> MAPKAKIVLVGSGMIGGVMATLIVQKNLGDVVLFDIVKNMPHGKALDTSHTNVMAYSNCKVSGSNTYDDLAGADVVIVTAGFTKAPGKSDKEANRDDLLPLNNKIMIEIGGHIKKNCPNAFIIVVTNPVDVMVQLLHQHSGVPKNKIIGLGGVLDTSRLKYYISQKLNVCPRDVNAHIVGAHGNKMVLLKRYITVGGIPLQEFINNKLISDAELEAIFDRTVNTALEIVNLHASPYVAPAAAIIEMAESYLKDLKKVLICSTLLEGQYGHSDIFGGTPVVLGANGVEQVIELQLNSEEKAKFDEAIAETKRMKALAHHHHHH

LDH and MDH are homologous, 2-ketoacid oxidoreductases that share both a protein fold (Rossmann et al., 1975) and a common catalytic mechanism (Birktoft and Banaszak, 1983; Clarke et al., 1986; Hart et al., 1987a, 1987b; Clarke et al., 1988; Waldman et al., 1988). Both enzymes are found in central metabolism: MDH catalyzes the interconversion of oxaloacetate and malate in the citric acid cycle, and LDH converts pyruvate to lactate in the final step of anaerobic glycolysis. A key event in the early evolution of the Apicomplexa was the acquisition of a malate dehydrogenase (MDH) via lateral gene transfer from α-proteobacteria. Following a gene duplication event roughly 700–900 Mya, one copy of this MDH evolved a novel substrate specificity to become a highly specific lactate dehydrogenase (LDH) that is now essential to the life cycle of many modern apicomplexans.

We tested the functional importance of residues in the specificity loop in PfLDH with an ‘alanine scan’ by individually mutating each residue in positions 101–108 to an alanine (note Ala103 was mutated to a serine). Mutating Trp107f to Ala reduced pyruvate activity by five orders of magnitude, whereas mutations at all other positions had effects less than a single order of magnitude, including the canonical specificity residue at position 102. The Trp107fAla mutation affects both kcat (1500-fold decrease) and Km (50-fold increase). To assess the effects of Trp107fAla mutation on the specificity loop conformation, we solved the crystal structure of PfLDH-W107fA (1.1 Å ) in the presence of oxamate and NADH. The protein crystallizes in the same space group as the wild-type PfLDH, with nearly identical cell dimensions. In the W107fA mutant, the specificity loop is disordered between residues Thr101 and Arg109, as is often seen in structures in which the loop is in the open conformation. In the mutant, residues 112–115 are in a linear α-helical conformation, in contrast to the wild-type PfLDH closed state which has a very prominent 60° kink in the α-helix at Pro114. Thus, the only significant difference between the wild-type and mutant structures is that the PfLDH-W107fA specificity loop is found in the open conformation, consistent with weaker binding of substrate. These results indicate that Trp107f is necessary for pyruvate activity in apicomplexan LDHs, and that it has become the new ‘specificity residue’ despite the fact that Trp107f does not align in sequence with the canonical specificity residue at position 102. Mutagenesis within the insertion indicates that only a single position, Trp107f, contributes strongly to pyruvate activity and specificity.> ANVRLQHHHHHHHLEAEAFSSESKWMTGDWGGTRTELLDKGYDFTLDYVGEVAGNLHGGYNDDKTARYSDQFALGAHLDLQKILGWHDAEFKLAITERSGRNLSNDRISDPRAGQFSSVQEVWGRGQTWRLTQMWIKQK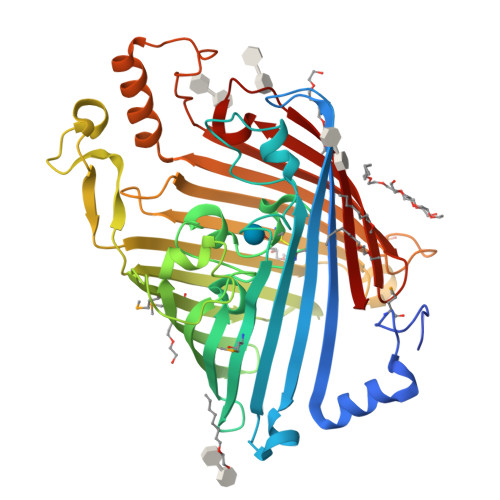YFDGALDVKFGRFGEGEDFNSFPCDFQNLAFCGSQVGNWVGGIWYNWPVSQWALRVKYNITPAFFVQVGAFEQNPSNLETGNGFKLSGSGTKGAIMPMEAVWSPKVNGLPGEYRLGYYYSTAKADDVYDDVNGNPQALTGEAFKSHSSKHGWWVVAQQQVTAHGGDVNRGLSLFANFTVHDKATNVVDNYQQVGLVYKGAFDARPKDDIGFGVARIHVNDDVKKRAELLNAQSGINDYDNPGFVPLQRTEYNAELYYGFHVTNWLTVRPNLQYIKSPGGVDEVDNALVAGLKIQSSF> MKTRTLKVLKPTLALLLAASFSAGALAQEVTLRLVSAFPENGIYVQRLLPWIAKVNAEGKGVLQINFLGGPKAIPTFEAGNAVKTGVVDMAMNTGAFYTNVMPEADFLKLTQIPVAEQRKNGAFDAINKVWNEKGNTQYLARMVENQPFHIYTNKKIDKPDLSGQKIRISPVYRDFFQALNANVVTTPPGEVYTALERGVVD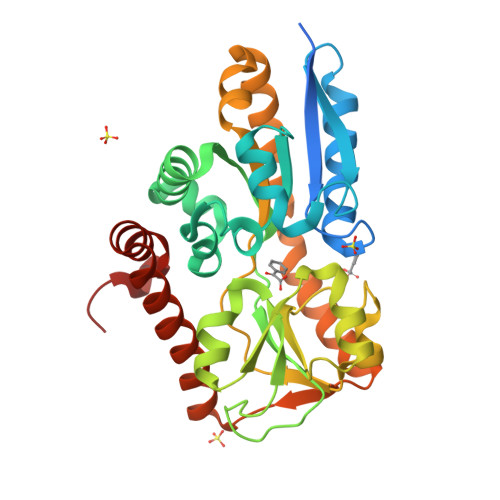GYGWPIGGIFDLNWQEKTKFRVDPGFYDAEVSLTMNLPAYKKLTDAQRNYLQKQLLVLEAENTFWTRYGNVETARQETAGIQTIKFDAATSKAFREKAYEVGWAGAMKQSPEVAARFKTLFSKAENLYFQ>GAMGSMPTYFDPIMQEDTVLDENTIVYLVKIGDNKFSIKAISSGLEHLPSDPTTHAEKYWPIPAKSLIDHSSNKLLFEEDKLTNQPISKDQVIELFAVD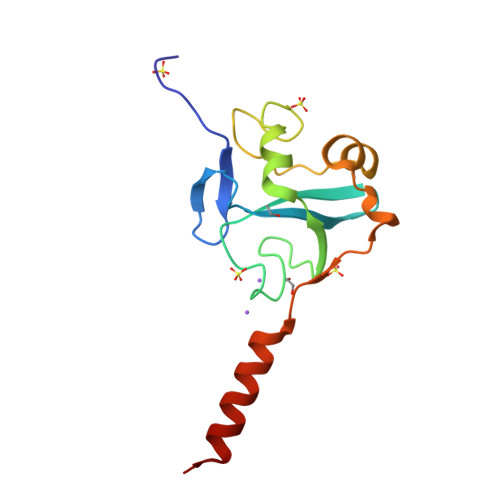PDKTEPKQFSDSVKRELTENWAREVLQDQ[3x]(4S,8E)-4-[(1R)-2-{[2-(5-tert-butyl-1,3-oxazol-2-yl)propan-2-yl]amino}-1-hydroxyethyl]-16-methyl-6-oxa-3-azabicyclo[12.3.1]octadeca-1(18),8,14,16-tetraene-2,13-dione | C29 H41 N3 O5 | 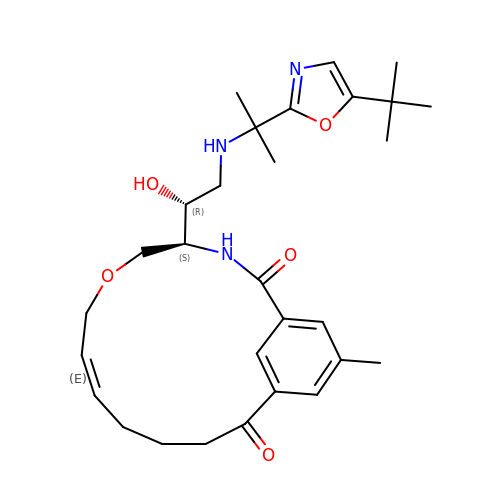PYRAVCNCGMDZRY-BDCWSOESSA-N> MQGVNIYNISAGTSVDLAAPVTTGDIVTFFSSAANLNAGAGNPNNTTLNLFAENGAYLLHIAFRLQENVIIFNSRQPDGPWLVEQRVSDVANQFAGIDGKAMVTVFDHGDKYQVVINEKTVIQYTKQ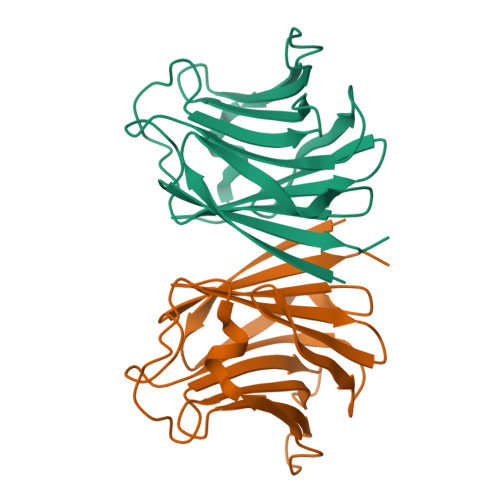ISGLTSSLSYNATEETSIFSTVVEAVTYTGLALEHHHHHH>[2x]GPGYQDPNNRYSFIGGRTGQWQVVKIRNVLGPGLQLVEKVNILNGAVAEIPLDSAWRLQGFASNIRYAIRTELEALQAVVPM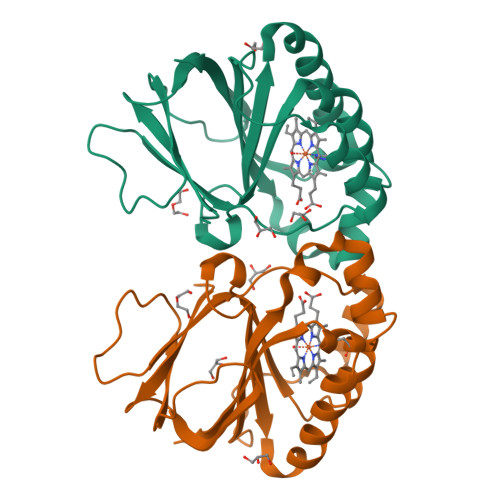LNRAEAILAVLIPIKKSAQWWEMAQDERRDIFERESHHTAVGLEYLPGVARRLLHCRDLGEEFDFLTWFEFAPEHSSAFNELLLRMRASKEWEYVEREVEVWLKRL> QSMQPRRVELWREPSKSLGISIVGGRGMGSRLSNGEVMRGIFIKHVLEDSPAGKNGTLKPGDRIVEVDGMD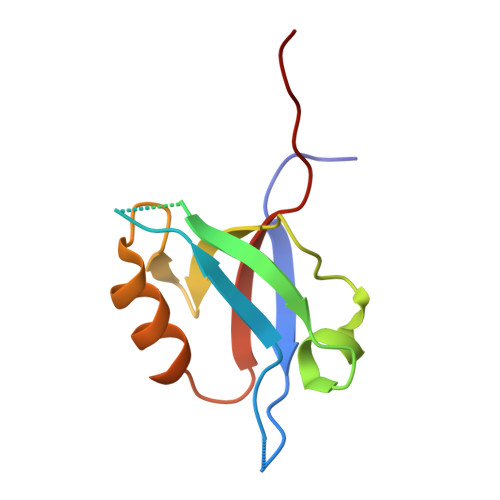LRDASHEQAVEAIRKAGNPVVFMVQSIISTRL> GSSRGIPPKIEALPSDISIDEGKVLTVACAFTGEPTPEVTWSCGGRKIHSQEQGRFHIENTDDLTTLIIMDVQKQDGGLYTLSLGNEFGSD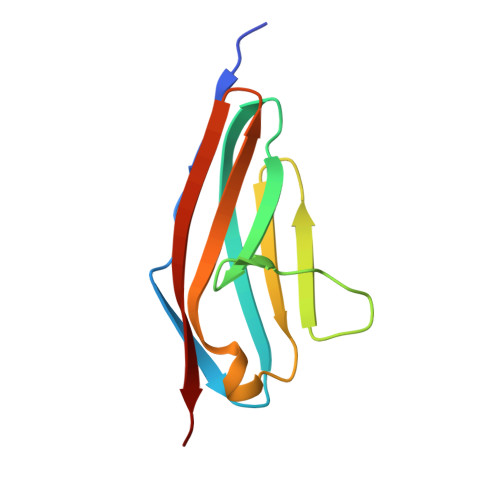SATVNIHIRSI>[6x]MTMIIGVYGASGFGKEVMPLVRQQFPTLSKEQFAFIDDGLSGTTLNGYPVLSYLDFISKPAD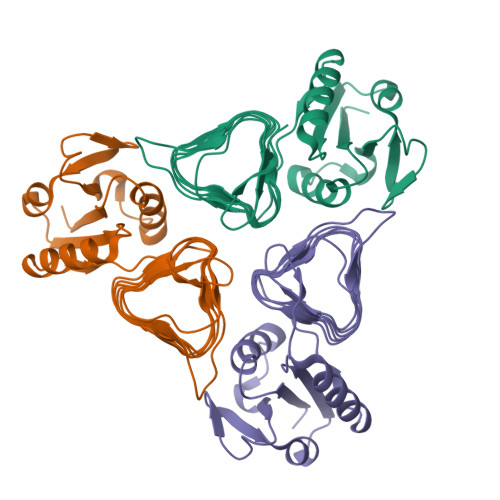HKAVTIAIANSVVREKLVSLLEKDGVQHLAVQSTNTVILDEVEIGEGSLLCPFTCLTSNIKIGKFFHANIYSYVAHDCVIGDYVTFAPGAKCNGNIHIEDHAYIGTGAVIKQGTPDKPLIIGKGAIVGMGAVVTKSVPAGVTVVGNPARILERK>MEFTTGLMSLDTALNEMLSRVTPLTAQETLPLVQCFGRILASDVVSPLDVPGFDNSAMDGYAV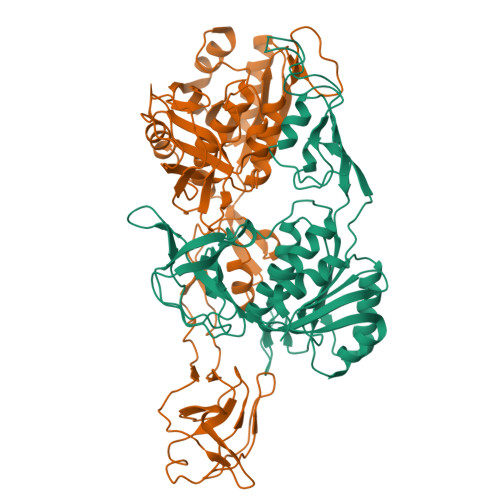RLADIASGQPLPVAGKSFAGQPYHGEWPAGTCIRIMAGAPVPEGCEAVVMQEQTEQMDNGVRFTAEVRSGQNIRRRGEDISAGAVVFPAGTRLTTAELPVIASLGIAEVPVIRKVRVALFSTGDELQLPGQPLGDGQIYDTNRLAVHLMLEQLGCEVINLGIIRDDPHALRAAFIEADSQADVVISSGGVSVGEADYTKTILEELGEIAFWKLAIKPGKPFAFGKLSNSWFCGLPGNPVSATLTFYQLVQPLLAKLSGNTASGLPARQRVRTASRLKKTPGRLDFQRGVLQRNADGELEVTTTGHQGSHIFSSFSLGNCFIVLERDRGNVEVGEWVEVEPFNALFGGL[2x]>[10x]TPDCVTGKVEYTKYNDDDTFTVKVGD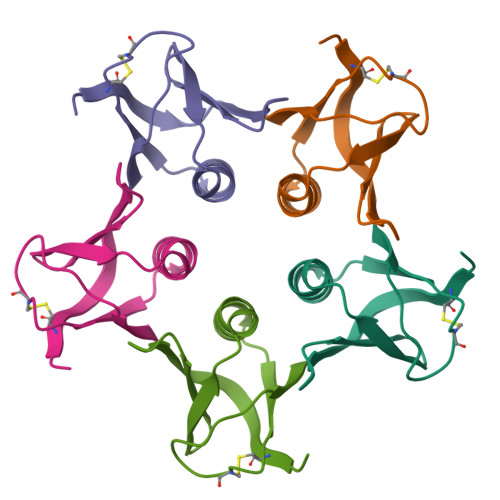KELFTNRANLQSLLLSAQITGMTVTIKTNACHNGGGFSEVIFR>[2x]MIGTQIVTERLVALLESGTEKVLLIDSRPFVEYNTSHILEAININCSKLMKRRLQQDKVLITELIQHSAKHKVDIDCSQKVVVYDQSSQDVASLSSDCFLTVLLG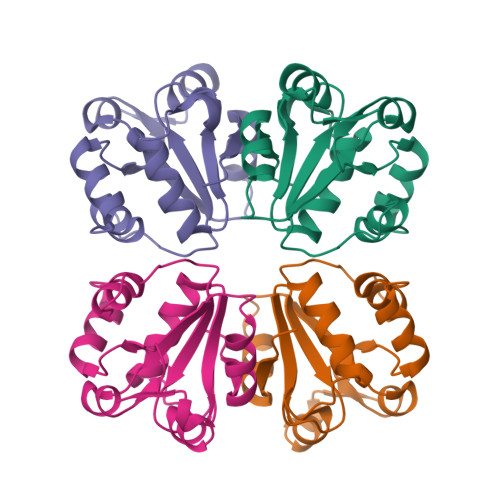KLEKSFNSVHLLAGGFAEFSRCFPGLCEGKSTLVPTCISQPAHHHHHH> ADNRPEKWVKGVCRYCGTGCGVLVGVKDGKAVAIQGDPNNHNAGLLCLKGSLLIPVLNSKERVTQPLVRRHKGGKLEPVSWDEALDLMASRFRSSIDMYGPNSVAWYGSGQCLTEESYVANKIFKGGFGTNNVDGNPRLCMASAVGGYVTSFGKDEPMGTYADIDQATCFFIIGSNTSEAHPVLFRRIARRKQVEPGVKIIVADPRRTNTSRIADMHVAFRPGTDLAFMHSMAWVIINEELDNPRFWQRYVNFMDAEGKPSDFEGYKAFLENYRPEKVAEICRVPVEQIYGAARAFAESAATMSLWCMGINQRVQGVFANNLIHNLHLITGQICRPGATSFSLTGQPNACGGVRDGGALSHLLPAGRAIPNAKHRAEMEKLWGLPEGRIAPEPGYHTVALFEALGRGDVKCMIICETNPAHTLPNLNKVHKAMSHPESFIVCIEAFPDAVTLEYADLVLPPAFWCERDGVYGCGERRYSLTEKAVDPPGQCRPTVNTLVEFARRAGVDPQLVNFRNAEDVWNEWRMVSKGTTYDFW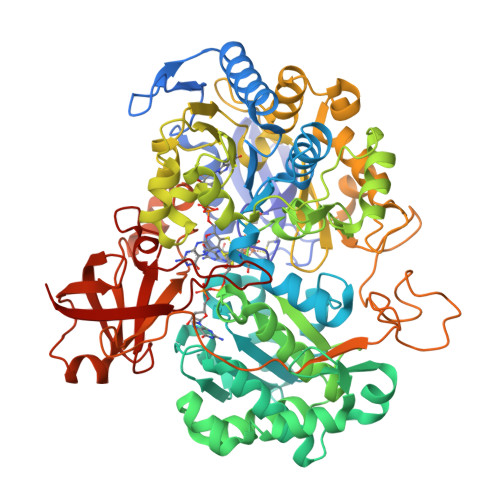GMTRERLRKESGLIWPCPSEDHPGTSLRYVRGQDPCVPADHPDRFFFYGKPDGRAVIWMRPAKGAAEEPDAEYPLYLTSMRVIDHWHTATMTGKVPELQKANPIAFVEINEEDAARTGIKHGDSVIVETRRDAMELPARVSDVCRPGLIAVPFFDPKKLVNKLFLDATDPVSREPEYKICAARVRKA> MAGNKPFNKQQAEPRERDPQVAGLKVPPHSIEAEQSVLGGLMLDNERWDDVAERVVADDFYTRPHRHIFTEMARLQESGSPIDLITLAESLERQGQLDSVGGFAYLAELSKNTPSAANISAYADIVRERAVVREMISVANEIAEAGFDPQGRTSEDLLDLAESRVFKIAESRANKDEGPKNIADVLDATVARIEQLFQQPHDGVTGVNTGYDDLNKKTAGLQPSDLIIVAARPSMGKTTFAMNLVENAAMLQDKPVLIFSLEMPSEQIMMRSLASLSRVDQTKIRTGQLDDEDWARISGTMGILLEKRNIYIDDSSGLTPTEVRSRARRIAREH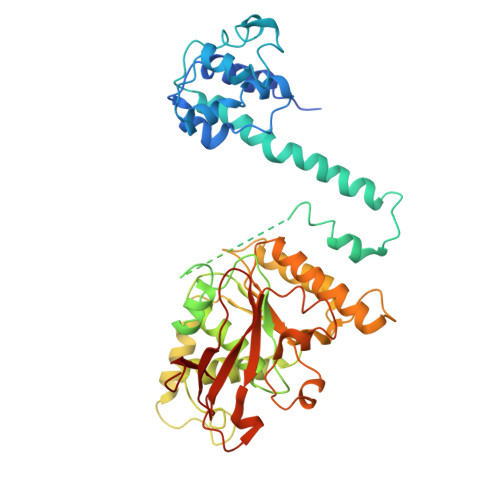GGIGLIMIDYLQLMRVPALSDNRTLEIAEISRSLKALAKELNVPVVALSQLNRSLEQRADKRPVNSDLRESGSIEQDADLIMFIYRDEVYHENSDLKGIAEIIIGKQRNGPIGTVRLTFNGQWSRFDNYAGPQYDDE1-Deoxy-d-xylulose 5-phosphate reductoisomerase from Plasmodium falciparum (PfDXR or PfIspC) is a homodimeric enzyme, with each subunit consisting of 488 amino acid residues. The enzyme DXR is also known as IspC, derived from the gene name ispC in the isoprenoid biosynthesis pathway. It is the enzyme responsible for the second step of a six-step catalytic reaction sequence catalyzing the conversion of the substrate 1-deoxy-d-xylulose 5-phosphate (DOXP) to 2-C-methyl-d-erythritol 4-phosphate (MEP) in the non-mevalonate pathway (MEP pathway). Accordingly, DXR, which belongs to the MEP pathway, a metabolic pathway not present in mammals, is regarded as a promising target for drug discovery. For the catalytic function of DXR, one molecule of NADPH and one divalent metal ion (either Mn2+ or Mg2+) are required per subunit as cofactors.

The N-phenylethyl group of MAMK150 adopted a curved conformation that did not fit into the subpocket. In the MAMK150 complex, the active site subpocket of PfDXR was occupied by five water molecules. Notable differences between the MAMK150 complex and the MAMK89 complex are that the MAMK150 complex exhibited a slightly more open loop structure, and the position of the side chain of Trp296 was completely different. In the case of the MAMK150 and MAMK251 complexes, the linker lengths are insufficiently long (ethyl) or excessively long (pentyl), respectively, and the phenyl moiety of the N-substituents is unable to utilize the subpocket. The reason for the significantly lower inhibitory activity of MAMK150 (64 nM) in comparison to those of MAMK89 (30 nM), MAMK218 (35 nM), and MAMK251 (29 nM) remains unclear based on the results of crystal structure analyses and computational analyses. With regard to the experimental observations, the side chain of Trp296 is in closer vdW contact with the side chains of Cys338 and Pro358 belonging to the active site core in the case of the MAMK150 complex when compared to the other complexes. This resulted in lower temperature factors and clearer electron densities for residues 291-299 being observed for the MAMK150–ternary and MAMK150–quaternary complexes. As an illustration, MAMK150 exhibits a markedly diminished capacity to inhibit PfDXR among the compounds under examination in this study. However, with regard to its capacity to inhibit the growth of P. falciparum, MAMK150 exhibits efficacy that is commensurate with that of MAMK89.

>[2x]MKKYIYIYFFFITITINDLVINNTSKCVSIERRKNNAYINYGIGYNGPDNKITKSRRCKRIKLCKKDLIDIGAIKKPINVAIFGSTGSIGTNALNIIRECNKIENVFNVKALYVNKSVNELYEQAREFLPEYLCIHDKSVYEELKELVKNIKDYKPIILCGDEGMKEICSSNSIDKIVIGIDSFQGLYSTMYAIMNNKIVALANKESIVSAGFFLKKLLNIHKNAKIIPVDSEHSAIFQCLDNNKVLKTKCLQDNFSKINNINKIFLCSSGGPFQNLTMDELKNVTSENALKHPKWKMGKKITIDSATMMNKGLEVIETHFLFDVDYNDIEVIVHKECIIHSCVEFIDKSVISQMYYPDMQIPILYSLTWPDRIKTNLKPLDLAQVSTLTFHKPSLEHFPCIKLAYQAGIKGNFYPTVLNASNEIANNLFLNNKIKYFDISSIISQVLESFNSQKVSENSEDLMKQILQIHSWAKDKATDIYNKHNSS>GAMDPASLEEMLTQAVQEADIEQVRQLLERGADANFQEEEWGWSPLHSAVQMDSEDLV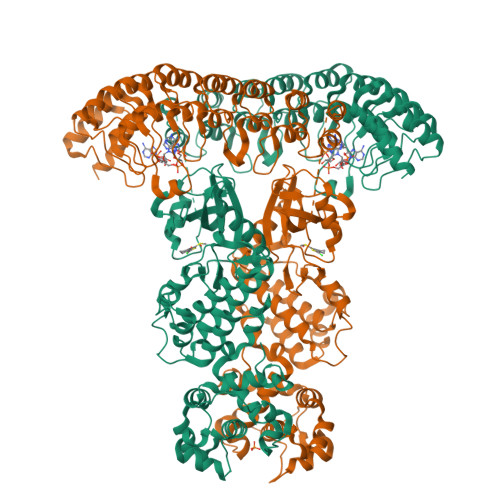ALLLKHGADPCLRKRNGATPFIIAGITGNVRLLQLLLPNVEDVNECDVNGFTAFMEAAVYGRVEALRFLYENGADVNMHRKTKQDQERIRKGGATALMDAAEKGHVGVVTILLHAMKAEVDARDNMGRNALVYALLNPDDGKAKAITRLLLDHGADVNVRGEGSKTPLILAVERKNLDLVQMLLEQEQIEVNDTDREGKTALLLAVELRLEEIAKLLCHRGASTNCGDLVAIARRNYDSDLVKFLRLHKAGEDFRPPAENWKPQSSRWGEALKHLHRIWRPMIGKLKIFIDEEYKIADTAEGGIYLGLYEDQEVAVKRFSEGSTRGQQEVSCLQSSRANDNVVTFYGSESDGSCLHVCLALCEYTLQEHLANHRGDAVPNEEDESARNILSSLFKAIGELHRSGYSHQDLQPQNILIDSKNGTFLADFDKSIKWAEDPQKIKRDLEALGLLVLYVVKKGDISFETLKNQSFEEVIQGSPDEETRDLIHHLFHPGDNVEDRLSSLLAHPFFWSWESRYRTLRDVGNESDIKTRNQNSRILQLLQPGTSELSTSFAQWTTKIDSFVMEEMNAYYKKISKKKKAKHTNEGNLYQDTLGDLLKFIRNLGEHINEQKNKKMKSIIGEPSQYFQEKFPDLVMYVYTKLQNTEYMKHFPKTHNPNK[2x]>WRCCQRVVGWVPVLFITFVVVWSYYAYVVELCVFTIFGNEENGKTVVYLVAFHLFFVMFVWSYWMTIFTSPASPSKEFYLSNSEKERY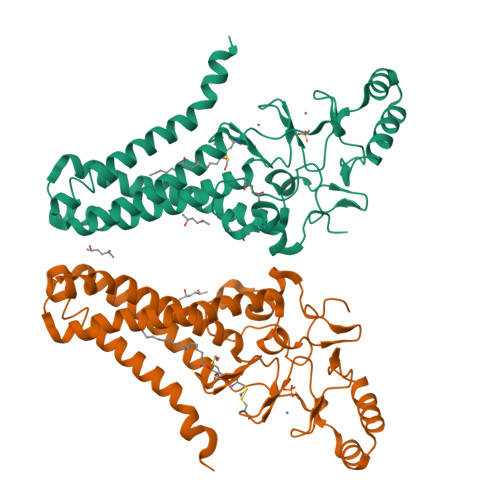EKEFSQERQQEILRRAARALPIYTTSASKTIRYCEKCQLIKPDRAHHCSACDSCILKMDHHCPWVNNCVGFSNYKFFLLFLLYSLLYCLFVAATVLEYFIKFWTNELTDTRAKFHVLFLFFVSAMFFISVLSLFSYHCWLVGKNRTTIESFRAPTFSYGPDGNGFSLGCSKNWRQVFGDEKKYWLLPIFSSLGDGCSFPTRLVGM[2x]>[4x]MASKPTLKEVVIVSATRTPI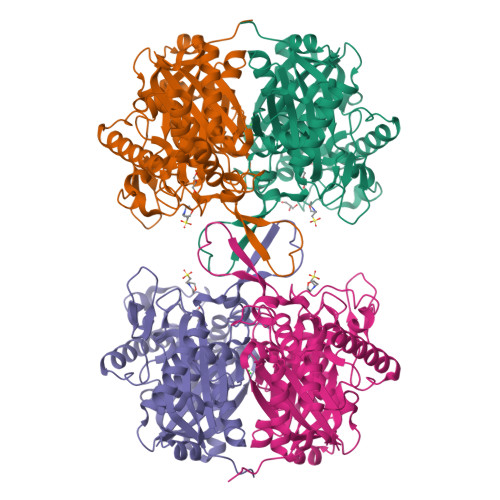GSFLGSLSLLPATKLGSIAIQGAIEKAGIPKEEVKEAYMGNVLQGGEGQAPTRQAVLGAGLPISTPCTTINKVCASGMKAIMMASQSLMCGHQDVMVAGGMESMSNVPYVMNRGSTPYGGVKLEDLIVKDGLTDVYNKIHMGSCAENTAKKLNIARNEQDAYAINSYTRSKAAWEAGKFGNEVIPVTVTVKGQPDVVVKEDEEYKRVDFSKVPKLKTVFQKENGTVTAANASTLNDGAAALVLMTADAAKRLNVTPLARIVAFADAAVEPIDFPIAPVYAASMVLKDVGLKKEDIAMWEVNEAFSLVVLANIKMLEIDPQKVNINGGAVSLGHPIGMSGARIVGHLTHALKQGEYGLASICNGGGGASAMLIQKL> TNAVNIVMRQPTTPNFSSALNITSANEGGSAMQIRGVEKALGTLKITHENPSVDKEYDENAAALSIDIVKKQKGGKGTAAQGIYINST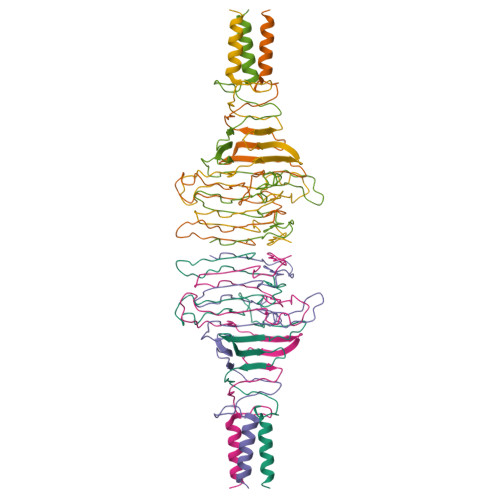SGTAGKMLRIRNKNKDKFYVGPDGDFWSCASSIVDGNLTVKDPTSGKHAATKDYVDEKIAELKKLILKK B cell lymphoma-2 (Bcl-2) antagonist/killer (Bak) is a critical executor of mitochondrial outer membrane permeabilization (MOMP), the key process of the type I programmed cell death called apoptosis. Bak is a member of the Bcl-2 protein family, which comprises 3 subgroups: proapoptotic BH3-only proteins, antiapoptotic Bcl-2 homologues, and downstream MOMP executors Bak and Bcl-2-associated X (Bax). Once activated, Bak and Bax undergo a conformational change to oligomerize on the mitochondrial membrane, which causes MOMP to be characterized by loss of mitochondrial membrane potential (ΔΨm) and release of cytochrome c. Pxt1, a male germ cell–specific protein exclusively expressed during spermatogenesis, was reported to contain a BH3 domain and to induce germ cell apoptosis and male mouse infertility upon overexpression.

Next, Bak(23–185;C166S) bound to human Pxt1(76–101) was subjected to crystallization, leading to structural determination of this complex to a resolution of 2.2 Å. In this complex structure, the human Pxt1 BH3 fragment forms an amphipathic α-helix and is accommodated in the BH3-binding groove of the single Bak molecule, similar to its binding to the corresponding region of Bcl-xL, with the equivalent positions of the 5 key BH3 consensus residues. With the lack of detergent treatment during the purification and crystallization steps, C-terminal helix swapping of Bak was not observed in our structure, which was reported to be induced by the combination of detergent and the BH3 fragment and necessary for the 2:2 complex form. The intermolecular binding between Bak and Pxt1 was mainly mediated by hydrophobic interactions: 4 hydrophobic BH3 consensus residues (Leu82, Leu86, Ile89, and Ile93) and 2 additional nonconserved isoleucine residues (Ile78 and Ile79) of human Pxt1 associate with Ile81, Gly82, Ile85, Tyr89, Phe93, Met96, Leu97, Leu100, Tyr110, Lys113, Ile114, Gly126, Val129, Ala130, Leu131, and Phe134 of Bak. We also found that Asp91, another conserved BH3 consensus residue in human Pxt1, contributes to complex formation by mediating electrostatic interactions with Arg127 and hydrogen bonding with Asn124 of Bak. The guanidinium group of Arg87 of Pxt1 also forms a hydrogen bond with the main-chain carbonyl of Ser117 of Bak. In the complex structure, a 310-helix between α2 and α3 (α2–α3 310-helix; residues 84–88) and the α3 helix (residues 89–100) of Bak containing the steric hindrance-associated residues are moved away toward the opposite side of α4, which widens the BH3-binding groove of Bak and enables the human Pxt1 BH3 domain to be accommodated in the pocket. Furthermore, binding of human Pxt1 BH3 induces the formation of a “cavity” in the middle of the BH3-binding groove of Bak, which was previously reported to reflect the conformational change of Bak or Bax induced by BH3 domain binding.

>[12x]GHMSEEQVAQDTEEVFRSYVFYRHQQEQEAEGVAAPADPEMVTLPLQPSSTMGQVGRQLAIIGDDINRRYDSEFQTMLQHLQPTAENAYEYFTKIATSLFESGINWGRVVALLGFGYRLALHVYQHGLTGFLGQVTRFVVDFMLHHSIARWIAQRGGWVAALNLGN;>GHMEEIIHKLAMQLRHIGDNIDHRMVRED[12x]>MRGLSRRVQAMKPDAVVAVNAKALELRRQGVDLVALTAGEPDFDTPEHVKEAARRALAQGKTKYAPPAGIPELREALAEKFRRENGLSVTPEETIVTVGGSQALFNLFQAILDPGDEVIVLSPYWVSYPEMVRFAGGVVVEVETLPEEGFVPDPERVRRAITPRTKALVVNSPNNPTGAVYPKEVLEALARLAVEHDFYLVSDEIYEHLLYEGEHFSPGRVAPEHTLTVNGAAKAFAMTGWRIGYACGPKEVIKAMASVSRQSTTSPDTIAQWATLEALTNQEASRAFVEMAREAYRRRRDLLLEGLTALGLKAVRPSGAFYVLMDTSPIAPDEVRAAERLL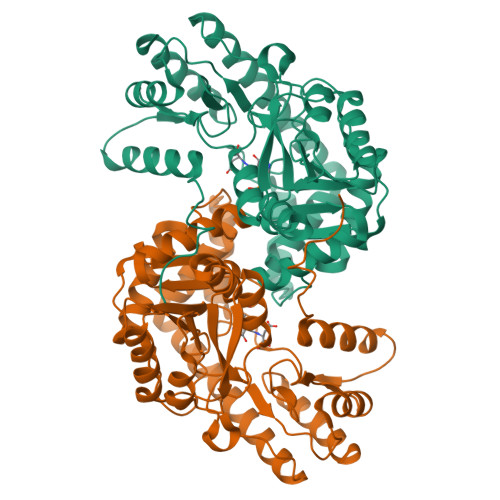EAGVAVVPGTDFAAFGHVRLSYATSEENLRKALERFARVLGRA[4x]> MEKKWWKEAVAYQIYPRSFMDSNGDGIGDIQGVISKLDYLSDLGIDV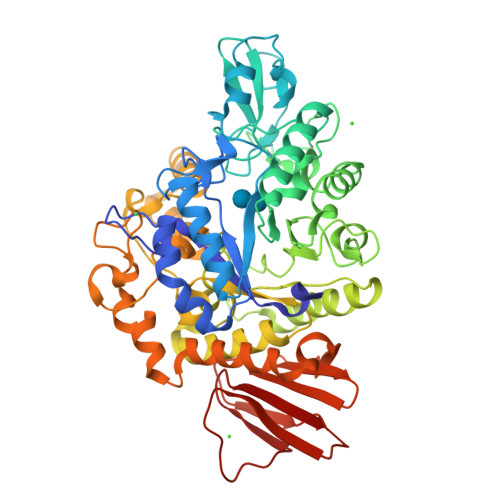IWICPIYQSPNDDNGYDISDYKDIMKDFGTMEDFDELLDEVHHRGMKLIMDLVINHTSDEHPWFLESRSAKENPYRDYYIWHEGKDGKEPNNWESIFSGSAWEFDEKTKEYYMHVFSKKQPDLNWENEKVRHELYEMVNWWLDKGIDGFRVDAISHIKKVAGFPDLPNPEKLDYVPSFEGHMNRPGIQEHLKELKEKTFAKYDIMTVGQANGVTSDSADEWVAEDGGNFNMIFQFEHMGLWDKGEEKPLDLIELKTILTNWQNGLEKINGWNALYLENHDQIRSVNKFGSTAYRVESAKCLAALYFLMKGTPFIYQGQELGMTNVKFDSIDDYDDVGMINYYRIQREKGDSHDEIMKVIWETGRDNSRTPMQWNTEKNAGFSTGNPWMKVNPNYVDINVEEQKSDKNSVLNFYKQLIKIRKQHDVLVYGTYKLLAEEDSAIYAYTRTLEGKTAVVICNMSPNNQTFEFPSESSFTNIEVLIHNYPLDKNETLEQCTLHPYETRVYLIS> TRDQNGTWEMESNENFEG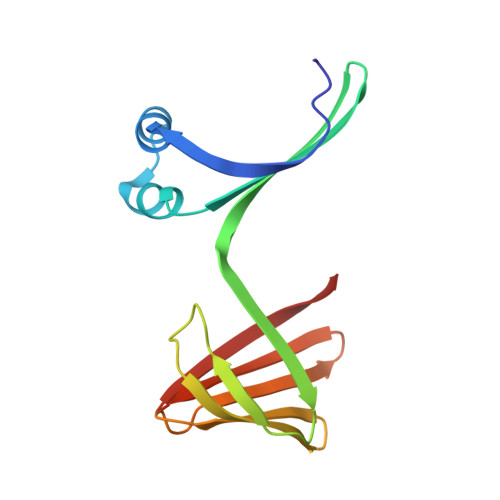YMKALDIDFATRKIAVRLTQTKVIDQDGDNFKTKTTSTFRNYDVDFTVGVEFDEYTKSLDNRHVKALVTWEGDVLVCVQKGEKENRGWKKWIEGDKLYLELTCGDQVCRQVFKKK>[2x]MARKYFVAANWKCNGTLESIKSLTNSFNNLDFDPSKLDVVVFPVSVH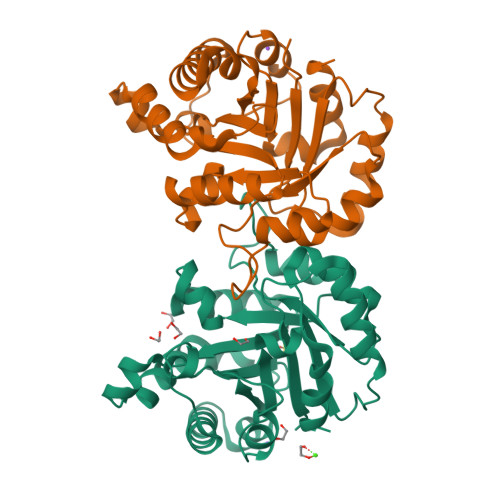YDHTRKLLQSKFSTGIQNVSKFGNGSYVGEVSAEIAKDLNIEYVIIGHFERRKYFHETDEDVREKLQASLKNNLKAVVCFGESLEQREQNKTIEVITKQVKAFVDLIDNFDNVILVYEPLWAIGTGKTATPEQAQLVHKEIRKIVKDTCGEKQANQIRILYGGSVNTENCSSLIQQEDIDGFLVGNASLKESFVDIIKSAM> MTIIEHGSLGTLPAPSVTTGIVDADIHPVPQDGALEPYLDDRWKKHIREYGVRTTTGLQFISEYPQMYGGAMRADAWPESGYPGSDRELLRTQLLDKHNIQLGVLQCLAPGGQTLNPAGQALNQELAAALCRATNDWQLEHL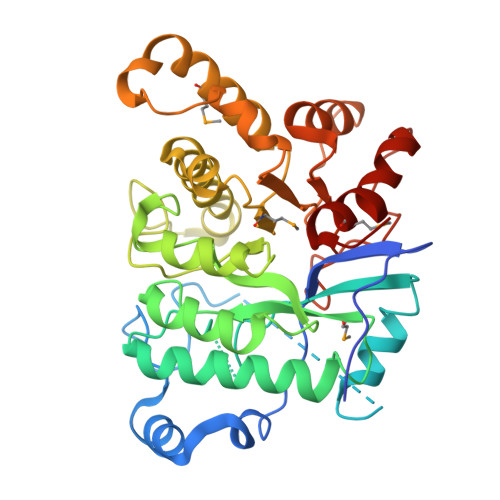VYPDPRMRAAIPVTFETPDYAVAEIERVGADPGVVAVLGTSKTLEPLGSRKYWPIYEASVAQNLPIQFHLSQGGGHANTGTGWTSYHTEYHTGHVQSFQSQLLSLVLSGTFDRFPTLKVMFVEGNVAHFAPLIQRMDYTWETLRGELPDLQRKPSEYIRDHIWASTQPIDEPEKPEHLAELLEEFCGDNVVFATDYPHFDFDDPETAFPRSFPVDLRDKILRGNGMRFFGVTNQAD2,4-DIAMINO-6-PHENYL-5,6,7,8,-TETRAHYDROPTERIDINE 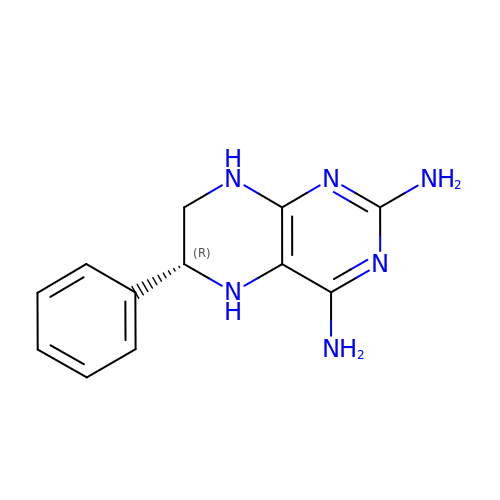| C12 H14 N6 | VEKRIXRQADJFAG-QMMMGPOBSA-N> GN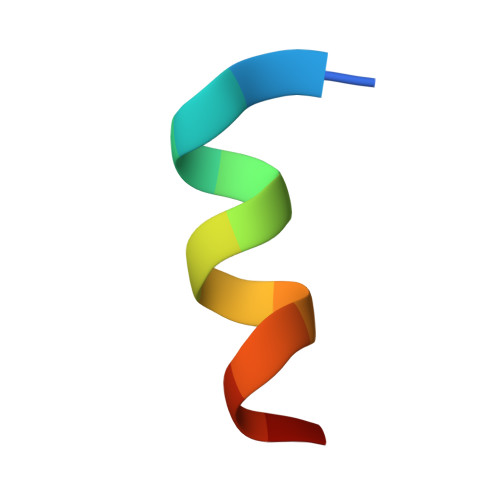SFDDWLASKGX>MKQLSTDAERELANIWATVLDIPIGTISASDNFFFRGGHSIDAMKASALGRAAGMSFGVADIFDHPVLSELASVAVA[8x];>KDSTESKSWEPFSLSPIKDPQALHKELCSKNVIPVTSTLEDLLPATQAQHVFIKRGTFHSYNWTIKGRSLNMDRLRETCQSLVDRHSILRTSFVEHEGHPIQLVLANLDVKVREVQCWPGEDPMEVCKALWDGKDWPTLNVLGGSLPVRFTLVSCPGNEHVVLTIQISHSQWDGVSIPKLFSDFAAIYNQTPLPPTSDFAHYLYHRVSSAREDVQQDPTFQFWRHYLDGAKMAVPFAPRALTLCAEPAAAAQSGQTLWTFKGIVPPTLPSGITMATLVKAATALFLSYHLGSRDVVFGHTVNGRNLPMDNIESLLGCTLNFVPLRVTFPEDSTDWTVMDLLHHTQTQYTRALSHEHVELRDIFQHSTNWPAETPLSLIVQHQNIDLSFSLPLRGSSVSGDGEDDSSLDVQYSKFARFDPLDEVWIFTEPHADRLEVQVCANSRVLGQEQATELANNISAIITKFSTDPTARLLD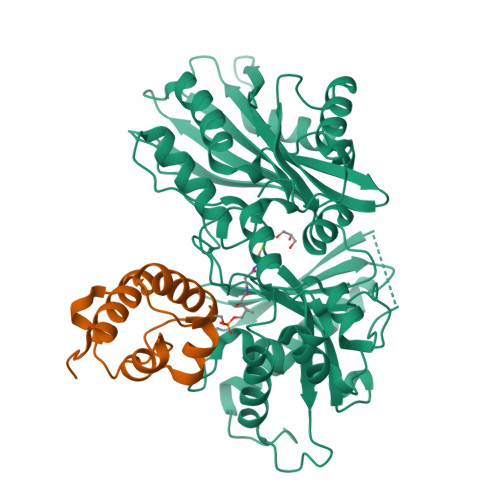ITF[8x]>[2x]GSGMQKLTILGATGSIGASTLKVIEQNPDKFS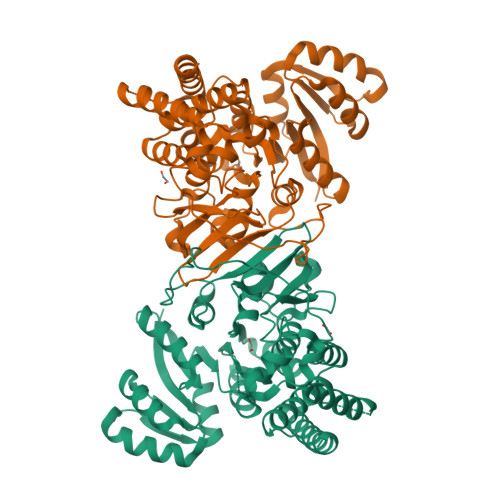VVALAADSNVEKMQQLCQRWQPEYAVMANKEAALRLKMALAVLAPNTQVLGGQEALCYVATLEQVDSVMAAIVGAAGLVPTMAAVKAGKRILLANKEALVMSGQLFIDEVEKSGAQLLPVDSEHNAIFQCLPQTVQGNLGRCDLASQGVSHILLTGSGGPFRYTDVAELEAVTPEQAIAHPNWSMGPKISVDSATMMNKGLEYIEAKWLFNASRDQLKVIIHPQSVIHSMVQYLDGSVLAQMGEPDMATPIALTLSYPERVKAGVKPLDFTQVGELTFLQPDFERYPCLALAIEACYLGQHATTTLNAANEVAVAAFLARQIKFTDIARVNDSVLNQVCKQSLASGLDSLESLLELDRMARTLADEVVRERAQ> MSNKVKTKAMVPPINCIFNFLQQQTPVTIWLFEQIGIRIKGKIVG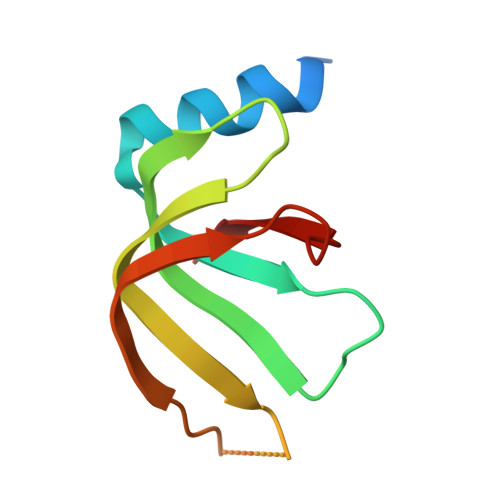FDEFMNVVIDEAVEIPVNSADGKEDVEKGTPLGKILLKGDNITLITSA> AAQTNAPWGLARISSTSPGTSTYYYDESAGQGSCVYVIDTGIEASHPEFEGRAQMVKTYYYSSRDGNGHGTHCAGTVGSRTYGVAKKTQLFGVKVLDDNGSGQYSTIIAGMDFVASDKNNRNCPKGVVASLSLGGGYSSSVNSAAARLQSSGVMVAVAAGNNNADARNYSPASEPSVCTVGASDRYDRRSSFSNYGSVLDIFGPGTDILSTWIGGSTRSISGTSMATPHVAGLAAYLMTLGKTTAASACRYIADTANKGDLSNIPFGTVNLLAYNNYQA;> PAPFA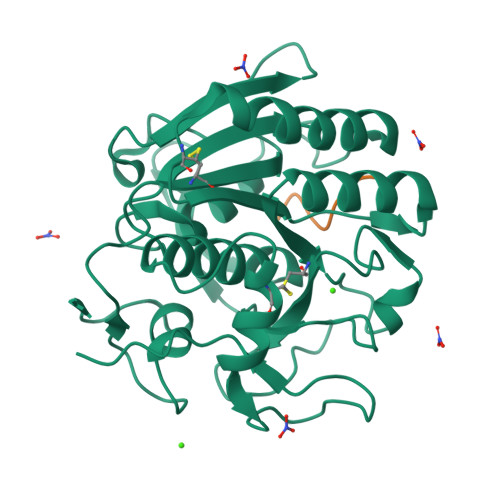SA> MEIPVIEPLFTKVTEDIPGAEGPVFDKNGDFYIVAPEVEVNGKPAGEILRIDLKTGKKTVICKPEVNGYGGIPAGCQCDRDANQLFVADMRLGLLVVQTDGTFEEIAKKDSEGRRMQGCNDCAFDYEGNLWITAPAGEVAPADYTRSMQEKFGSIYCFTTDGQMIQVDTAFQFPNGIAVRHMNDGRPYQLIVAETPTKKLWSYDIKGPAKIENKKVWGHIPGTHEGGADGMDFDEDNNLLVANWGSSHIEVFGPDGGQPKMRIRCPFEKPSNLHFKPQTKTIFVTEHENNAVWKFEWQRNGKKQYCETLKFGIF

The diisopropyl fluorophosphatase (DFPase) from the squid Loligo vulgaris is able to detoxify a broad range of organophosphorous compounds, including tabun, sarin and soman although its favorite substrate remains the diisopropyl fluorophosphate. The DFPase is a 35 kDa calcium-dependent enzyme that exhibits a six-bladed ß-propeller structure with two calcium ions in a central water-filled tunnel, similar to that of the mammalian recombinant paraoxonase-1. Blum et al. elicited the following mechanism based on a H218O isotope labeling experiment: the calcium-coordinated Asp_229 was identified as the nucleophile that attacks the phosphorus center of the substrate via the formation of a phosphoenzyme intermediate. Another possible catalytic mechanism for DFPase might involve the activation of a water molecule, as in PTEs, PLLs, human paraoxonase-1, and the lactonase from Staphylococcus aureus (drug resistance protein 35), a DFPase structural homologue.

After refinement, the R and Rfree factors of the DFPase X-ray model improved from 11.1 and 12.8% initially, down to 10.3 and 12.1%, respectively. Out of the 481 water molecules in the DFPase structure, the positions of hydrogen atoms of 20 water molecules could be established solely on account of electron density peaks. The small fraction of water molecules for which hydrogen atoms are visible interestingly comprise active site water molecules, thereby allowing us to construct unequivocally, the hydration shell and the water hydrogen-bond network in the DFPase central tunnel. The hydrogen bond network of water molecules is different in the X-N and X-ray structures, despite the similar localization of water oxygen atoms. In addition, the donor-acceptor (H…O) distances turn out to be shorter in the X-ray structure than in the X-N model. In the X-ray structure, a strong electron density peak (maximum contour: 4σ) is visible close to the equivalent water molecule (HOH_524), which can be unambiguously allocated to one of its hydrogen atom. Moreover, this electron density peak displays an elliptical shape, whereas all the other electron density peaks revealing water hydrogen atoms in the DFPase X-ray structure are spherical. The analysis of the chemical environment of the water molecule in the X-ray structure shows that HOH_524 is involved in the following interactions: (i) Its hydrogen atom, located with a strong electron density peak described earlier, points towards HOH 511 and forms a canonical hydrogen bond (Ow…Ow distance: 2.82 Å, angle Ow-Hw…Ow = 136°). (iii) The oxygen atom of HOH_524 is coordinated to the catalytic calcium (distance: 2.5 Å) and (iv) further interacts with the carboxylate side chain of Asp_229. Our investigation into the DFPase active site in the X-ray structure suggests that the calcium-coordinated water molecule HOH_524 is partially activated into a hydroxide ion through proton relocation towards the nearby Asp_229 Oδ2 atom.> GPMVTVTYDPSNAPSFQQEIANAAQIWNSSVRNVQLRAGGNADFSYYEGNDSRGSYAQTDGHGRGYIFLDYQQ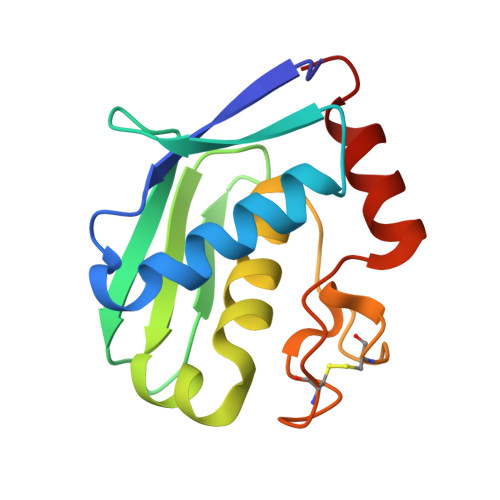NQQYDSTRVTAHETGHVLGLPDHYQGPCSELMSGGGPGPSCTNPYPNAQERSRVNALWANG>[2x]MTSRVDPANPGSELDSAIRDTLTYSNSPVPNALLTASESGFLDAAGIELDVLSGQQGTVHFTYDQPAYTRFGGEIPPLLSEGLRAPGRTRLLGITPLLGRQGFFVRDDSPITAAADLAGRRIGVSASAIRILRGQL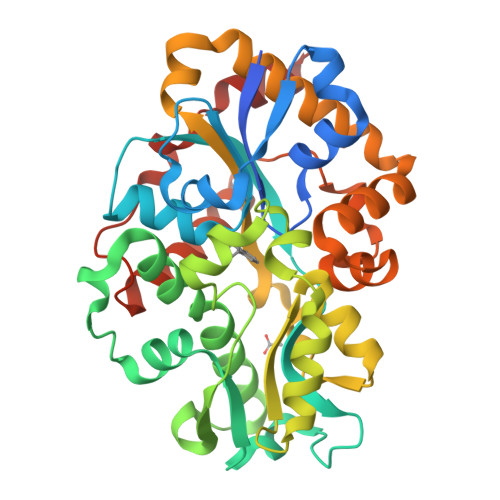GDYLELDPWRQTLVALGSWEARALLHTLEHGELGVDDVELVPISSPGVDVPAEQLEESATVKGADLFPDVARGQAAVLASGDVDALYSWLPWAGELQATGARPVVDLGLDERNAYASVWTVSSGLVRQRPGLVQRLVDAAVDAGLWARDHSDAVTSLHAANLGVSTGAVGQGFGADFQQRLVPRLDHDALALLERTQQFLLTNNLLQEPVALDQWAAPEFLNNSLNRHR> GQRGVVGLPGQ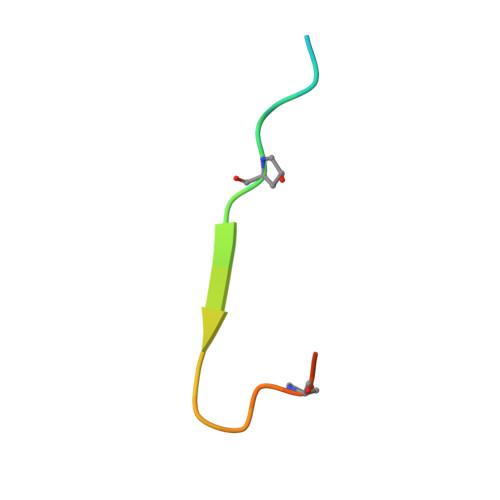RGERGFPGLPGY Based on primary and tertiary structure, the H. orenii glycosidase is a member of family 43 of inverting glycoside hydrolases, with accession No. cl14647 and sequence cluster cd08772 (superfamily GH43_62_32_68) in the Conserved Domains Database (CDD). The enzyme folds as a five-bladed β-propeller similar to those described for inverting GH43 enzymes of clan GH-F. Each blade is composed of a four-stranded antiparallel β-sheet repeated five times from the N-terminus to the C-terminus: blade 1, residues 14–59; blade 2, residues 69–120; blade 3, residues 125–179; blade 4, residues 190–244; blade 5, residues 255–306. The conserved catalytic nucleophile is placed on blade 4 (Glu195), the catalytic base (Asp17) on blade 1 and Asp126 on blade 3. The enzyme displays activity with pNP-αAraf as a substrate, but no detectable activity on pNP-αXyl or pNP-βXyl, which suggests that it is an α-1,5-l-arabinofuranosidase and not an α- or β-xylosidase.

The crystal structure of the H. orenii glycosidase was determined by molecular replacement and refined at 1.10 Å resolution. The deposited model includes riding H atoms, and the asymmetric unit contains two protein molecules (molecule A, residues 4–315; molecule B, residues 3–315), three HEPES molecules (one associated with molecule A and two with molecule B), one sodium ion per protein molecule and 1032 water molecules. As inferred from homology to related GH43 enzymes, the catalytic −1 subsite is situated at the bottom of a pocket formed at the ‘top’ of the β-propeller. On one side of the −1 subsite, Trp72 (blade 2) forms a conserved sugar-binding platform. In the present structure, the piperazine ring of the HEPES buffer molecule is wedged between Trp72 and Tyr215 in subsite −1, but does not form a planar stacking interaction with the aromatic rings. A metal-binding site is situated at the central axis of the propeller, immediately below the −1 subsite. The metal ion present in the structure is represented by a 20σ peak in the σA-weighted difference Fourier map with coordination to five ligands: Glu75 O∊2 (2.1 Å) and four water O atoms. The imidazole group of the nearby His256 (blade 5) is positioned as a possible sixth ligand, but is 2.8 Å from the metal ion. Thus, based on the composition of the crystallization medium, the observed coordination number and the metal–ligand coordination distances for the bound metal, we modelled the metal ion as Na+. The metal-binding site in the H. orenii GH43 glycosidase is strategically positioned at the propeller axis to provide stabilizing interactions between blade 2 (Glu75) and blade 5 (His256) across the axis, which probably explains the increase in melting temperature in the presence of divalent cations.

>[2x]MKDTYTNPVGGITGIGDPYVLKHESRYYLYATSAINRGFKVWESPNLVDWELKGLALDSYYEKNGWGTEDFWAPEVIFYNNKFYMTYSARDNDGHLKIALASSKSPLGPFKNIKAPLFDRGLSFIDAHIFIDQDGTPYIYYVKDCSENIINGIHISQIYVQEMSQDLLELKGDPVLAIQPSQDWEGINDAWQWNEGPFVIKHEGKYYMMYSANCYASPDYSIGYAVAETPLGPWIKYSGNPILSKRMDKGISGPGHNSVTVSPDGSELFVVYHTHTYPDSPGGDRTVNIDRLYFEDGILKVKGPTRSPQPGPRSN> MANVDEYITQLPAGANLALMVQKVGASAPAIDYHSQQMALPASTQKVITALAALIQLGPDFRFTTTLETKGNVENGVLKGDLVARFGADPTLKRQDIRNMVATLKKSGVNQIDGNVLIDTSIFASHDKAPGWPWNDMTQCFSAPPAAAIVDRNCFSVSLYSAPKPGDMAFIRVASYYPVTMFSQVRTLPRGSAEAQYCEL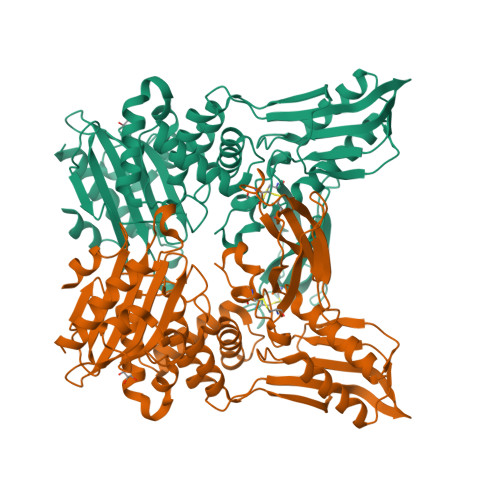DVVPGDLNRFTLTGCLPQRSEPLPLAFAVQDGASYAGAILKYELKQAGITWSGTLLRQTQVNEPGTVVASKQSAPLHDLLKIMLKKSDNMIADTVFRMIGHARFNVPGTWRAGSDAVRQILRQQAGVDIGNTIIADGSGLSRHNLIAPATMMQVLQYIAQHDNELNFISMLPLAGYDGSLQYRAGLHQAGVDGKVSAKTGSLQGVYNLAGFITTASGQRMAFVQYLSGYAVEPADQRNRRIPLVRFESRLYKDIYQNN>SMRKTIERLLNSELSSNSIAVRTGVSQAVISKLRNGKKELGNLTLNSAEKLFEYQKEMEKVDTWIVYRGRTADMNKSYIAEGSTYEEVYNNFVDKYGYDVLDEDIYEIQLLKKNGENLDDYDVDSDGINNYDKLDEFR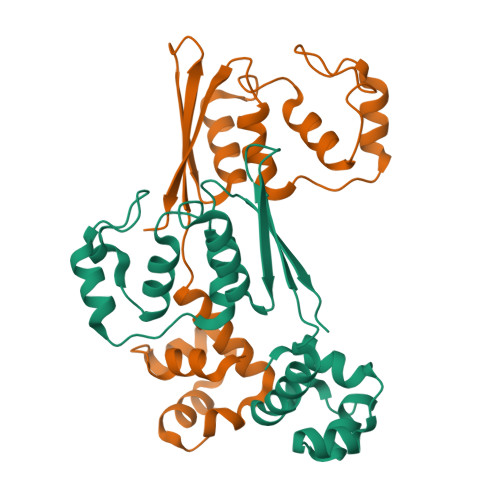ESDYVDLEDYDYRELFENSSSQVYYHEFEITHE[4x]>[4x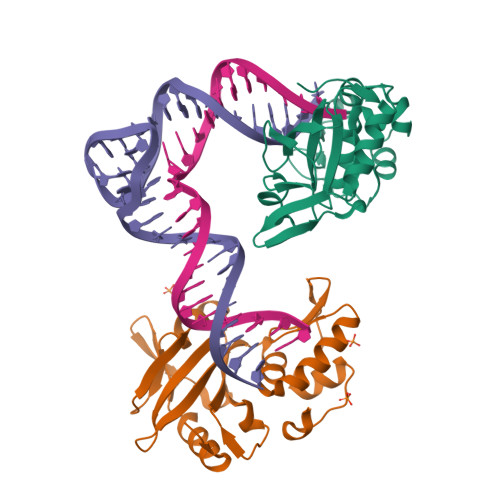]GGSMLTLIQGKKIVNHLRSRLAFEYNGQLIKILSKNIVAVGSLRREEKMLNDVDLLIIVPEKKLLKHVLPNIRIKGLSFSVKVCGERKCVLFIEWEKKTYQLDLFTALAEEKPYAIFHFTGPVSYLIRIRAALKKKNYKLNQYGLFKNQTLVPLKITTEKELIKELGFTYRIPKKRL> SLQPLPPTAFTPNGTYLQHLARDPTSGTLYLGATNFLFQLSPGLQLEATVSTGPVL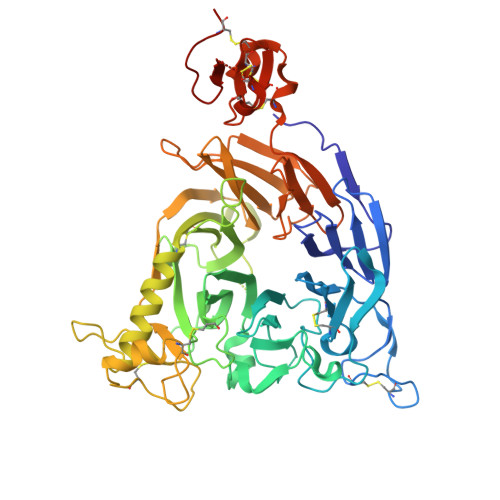DSRDCLPPVMPDECPQAQPTNNPNQLLLVSPGALVVCGSVHQGVCEQRRLGQLEQLLLRPERPGDTQYVAANDPAVSTVGLVAQGLAGEPLLFVGRGYTSRGVGGGIPPITTRALWPPDPQAAFSYEETAKLAVGRLSEYSHHFVSAFARGASAYFLFLRRDLQAQSRAFRAYVSRVCLRDQHYYSYVELPLACEGGRYGLIQAAAVATSREVAHGEVLFAAFSSAAPPTVGRPPSAAAGASGASALCAFPLDEVDRLANRTRDACYTREGRAEDGTEVAYIEYDVNSDCAQLPVDTLDAYPCGSDHTPSPMASRVPLEATPILEWPGIQLTAVAVTMEDGHTIAFLGDSQGQLHRVYLGPGSDGHPYSTQSIQQGSAVSRDLTFDGTFEHLYVMTQSTLLKVPVASCAQHLDCASCLAHRDPYCGWCVLLGRCSRRSECSRGQGPEQWLWSFQPELGCLQTRENLYFQ> MGKGHHHHHHGSERTGTQPLGVQGLTEEQRMMIRELMDAQMKTFDTTFSHFKNFRLPGVLSSGCELPESLQAPSREEAAKWSQVRKDLCSLKVSLQLRGEDGSVWNYKPPADSGGKEIFSLLPHMADMSTYMFKGIISFAKVISYFRDLPIEDQISLLKGAAFELCQLRFNTVFNAETGTWECGRLSYCLEDTAGGFQQLLLEPMLKFHYMLKKLQLHEEEYVLMQAISLFSPDRPGVLQHRVVDQLQEQFAITLKSYIE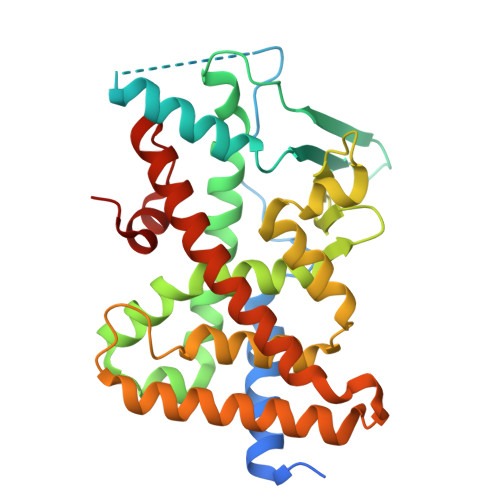CNRPQPAHRFLFLKIMAMLTELRSINAQHTQRLLRIQDIHPFATPLMQELFGITGS>[4x]AETVSFNFNSFSEGNPAINFQGDVTVLSNGNIQLTNLNKVNSVGRVLYAMPVRIWSSATGNVASFLTSFSFEMKDIKDYDPADGIIFFIAP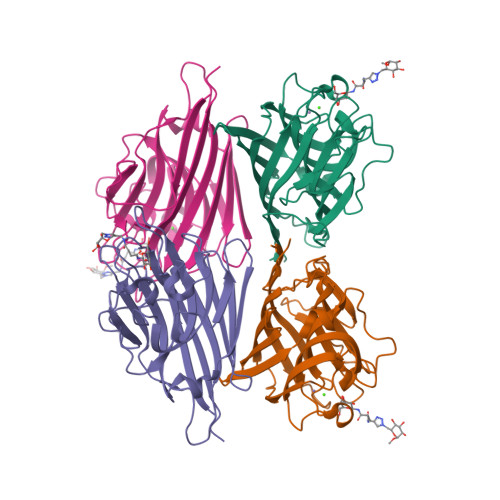EDTQIPAGSIGGGTLGVSDTKGAGHFVGVEFDTYSNSEYNDPPTDHVGIDVNSVDSVKTVPWNSVSGAVVKVTVIYDSSTKTLSVAVTNDNGDITTIAQVVDLKAKLPERVKFGFSASGSLGGRQIHLIRSWSFTSTLITTTRRS> XEKIAAIKEEQAAIEEEIQAIKEEI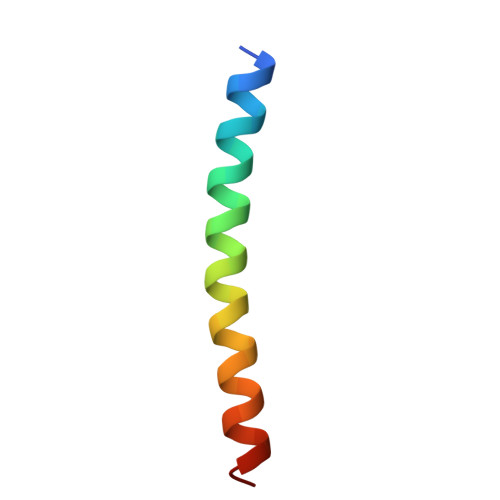AAIKYLIAQIX>[4x]KGKLPPVYPVTVPILGHIIQFGKSPLGFMQECKRQLKSGIFTINIVGKRVTIVGDPHEHSRFFLPRNEVLSPREVYSFMVPVFGEGVAYAA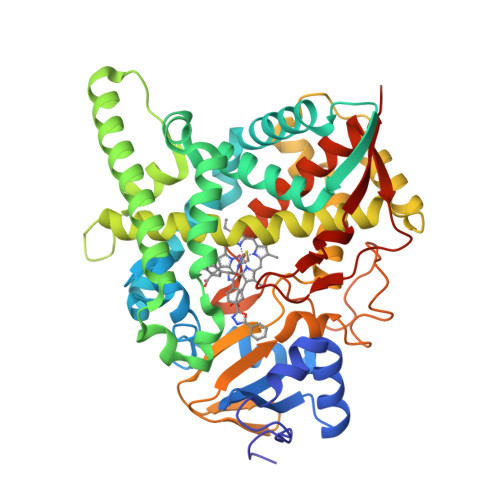PYPRMREQLNFLAEELTIAKFQNFVPAIQHEVRKFMAANWDKDEGEINLLEDCSTMIINTACQCLFGEDLRKRLDARRFAQLLAKMESSLIPAAVFLPILLKLPLPQSARCHEARTELQKILSEIIIARKEEEVNKDSSTSDLLSGLLSAVYRDGTPMSLHEVCGMIVAAMFAGQHTSSITTTWSMLHLMHPANVKHLEALRKEIEEFPAQLNYNNVMDEMPFAERCARESIRRDPPLLMLMRKVMADVKVGSYVVPKGDIIACSPLLSHHDEEAFPEPRRWDPERDEKVEGAFIGFGAGVHKCIGQKFGLLQVKTILATAFRSYDFQLLRDEVPDPDYHTMVVGPTASQCRVKYIRRK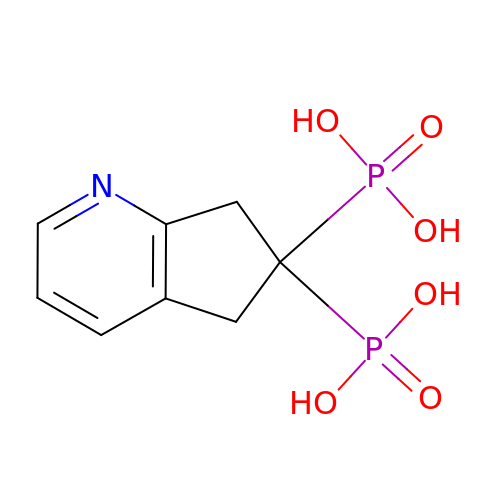6,7-dihydro-5H-cyclopenta[b]pyridine-6,6-diylbis(phosphonic acid) | C8 H11 N O6 P2 | BKUBDCZNHKIXPI-UHFFFAOYSA-N N-{3-[(3-{4-[(4-methoxyphenyl)amino]-1,3,5-triazin-2-yl}pyridin-2-yl)amino]-4-methylphenyl}-3-(trifluoromethyl)benzamide 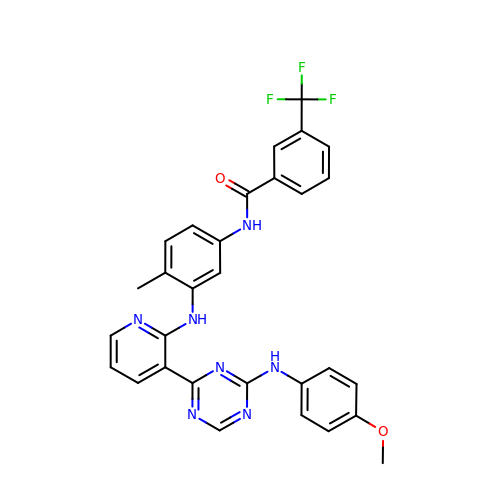| C30 H24 F3 N7 O2 | FLZNVZVIUIDCOF-UHFFFAOYSA-N>[2x]MSLGTYVPGDITLVDSYGNEFQLKNLKGKPIILSPIYTHCRAAC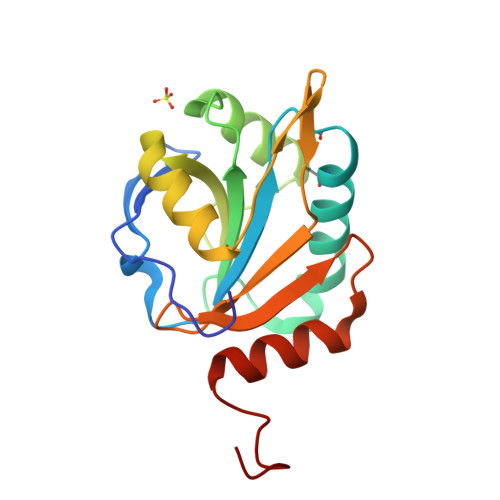PLITKSLLKVIPKLGTPGKDFWVITFTFDPKDTLEDIKRFQKEYGIDGKGWKVVKAKTSEDLFKLLDAIDFRFMTAGNDFIHPNVVVVLSPELQIKDYIYGVNYNYLEFVNALRLARGEGHHHHHH TRIFLUOROETHANOL | C2 H3 F3 O | 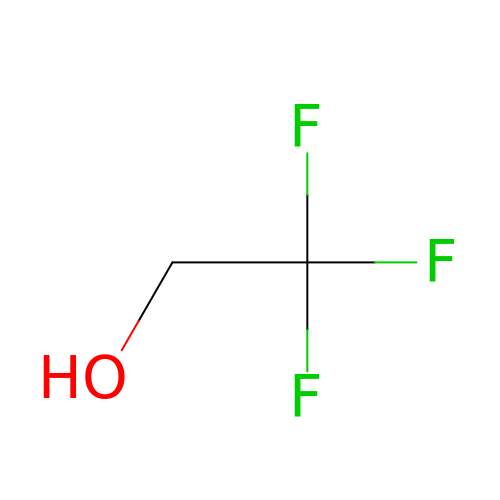RHQDFWAXVIIEBN-UHFFFAOYSA-N>VSSRVSTRSSLAEDLRAIGLADGDAVLVHAALRKVGKIVGGPDDILDAMRDVIGPAGTVLGYADWQLEDEIRDDPAMREHIPAFDPLRSRSIRDNGFWPELIRTTPGAL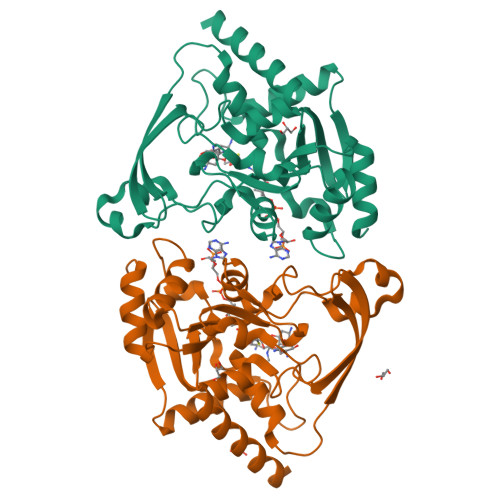RSASPGASMAAIGGEAEWFTADHALDYGYGPRSPLGKLVEAKGKVLMLGAPLDTMTLLAHAEHLADFPNKRILRYEAPILVDGEKVWRWFEEFDTSDPPDGLADDYFAGIVEEFLATGRGKRGKIGEASSVLVPADEIVAFAVDWLERWGRTAR[2x]Kinesins are a family of microtubule-based motors that play important roles in intracellular transport and cell division. Kinesin-1 transports cargo within cells, a process tightly coupled with ATP hydrolysis. Whereas kinesin-1 in solution is mostly loaded with ADP, ADP release is accelerated several thousand-fold upon microtubule binding. Here we characterized kinesin-1 P-loop mutations that interfere with ADP binding and determined the structure of the corresponding mutated nucleotide-free kinesins.

We were also able to crystallize in the same buffer conditions the nucleotide-free parental kinesin-1 (without the T92V mutation), following nucleotide digestion with apyrase, and to determine its structure. Remarkably this structure is isomorphous to that of ADP-kinesin10. Therefore, an ADP-kinesin-like conformation can be adopted both by nucleotide-free wild-type kinesin and by the T92V mutant. In contrast, the temperature factors of the P-loop are much closer to those of the central β-sheet both in ADP-kinesin10 and in apo-kinesin in an ADP-kinesin-like conformation (this work). Whereas we demonstrated that, in the absence of microtubules, apo-kinesin-1 may adopt two conformations, ADP-kinesin-like and tubulin-bound apo-kinesin-like, the effect of tubulin binding is to shift the balance between them and to stabilize the tubulin-bound apo-kinesin-like conformation, from which ADP is released and which is primed to bind ATP6.

> MADLAESNIKVMCRFRPLNESEVNRGDKYIAKFQGEDTVVIASKPYAFDRVFQSSTSQEQVYNDAAKKIVKDVLEGYNGTIFAYGQTSSGKTHTMEGKLHDPEGMGIIPRIVQDIFNYIYSMDENLEFHIKVSYFEIYLDKIRDLLDVSKTNLSVHEDKNRVPYVKGATERFVSSPDEVMDTIDEGKSNRHVAVTNMNEHSSRSHSIFLINVKQENTQTEQKLSGKLYLVDLAGSEKVSKTGAEGAVLDEAKNINKSLSALGNVISALAEGSTYVPYRDSKMTRILQDSLGGNARTTIVICCSPSSYNESETKSTLLFGQRAKTI> MADGPSPIRIVLWNDGGESLAAGVEDEEQQQVLHSFADLVGSAIDAVLELPQFRHVEAVTAEAEEDEPGLSIGFDAGSGDGEVDIDNLKGRLDIAGLLLGSAQLPEELAEVAAVEVTDEEEGTTELQFTDEGLVQQLQAVVKRAKLEKRYNDWVAGVAESLGPALDAAAGGVEVTEMPVDPYDVLQAVVAQLIRVAGVSPPAPSLFSRTGALVGGVLGAPRSAVRQVTKRLGRAQRLWWRLEDVVVDGSKLALRLAVKAARPVLVGFVLHRVLKTLDRSRQLEYRLARMGPEEAREAYYEAVLGKDWKQQLQADWDKALEDVDAGLVTDEINHEKRLMTAAQLRRLEVEEWDKQRMKNFYLASFGGLRWFDQMEQALHNPLFIESRGWTDPVQNWVGQNRTYMDDLPAGQYMAGVGNAAIRIKEAELKRKLTDVERAHVLARGGAVAGGLLPQQPTDPATLAVAVGGAFVPSVAGKR;> MGASQESELDFVPRLSFLPIEWRSIGSAFGLKDKSGAAANGRATFTVRQGVDAAELTSTGRVIDGQADVGASLKLNTLAIGVSASNITFHSGLDDPTAAAAQRSSLIPSLKLTAAKQFKRDNYIAVSYDLKHQKPELSACWTGEAGADRATLLVNVDPVMRSVKLAAAVRTPGPEWRKVLYNDETDLLEYPADDGARHTLYVQHEVRGRDLLHATRLGCRLDLGRLVNYVVDFVDYRIEENIPSFVWNVPLLPQLYSLLVPADNDEQVRHRITGWELDVSHDFARSGLLPVVAISKTSKKLLGGGTLTASYDAAAREAGVSLSRKGVSVGARVARAEGAAGGLSAGWGRPSIHVAVEPLGLLQ;> MQLGQLRQPLRACQDQRLTRGVPLARRQLVVVSNWNPLGGKGGGNAEQPGGEEPIQDELLKLLRGGWVLLSNLALFLVFSSFLHRSLNWFVQTELLVAVGAPQQAGERVVGKFFEAIEWVERNILGWKLPGDEEAEDATSKVYEVLQNYTPAEAAYSFAQLKYKDLTHKERELFHKAYALRHFERRDGRPGDVDAAELQAVKDRLDPLEADRRAYAAAKAAGRLDEYWAAPGREATYQRIVGAPRIAARQCEMASMLKGLQAVLPAMELLAQLQVAQFVYAASKASKSRQQDDFKLQLQTFYGNVLDEQCQLRCMLLNVQLPMALVTVFVPQYCFCLLDRVVLPRRECGSASTLGSLLRACGRPGSACHAGGCSAQRRDPLTI;> MQGLKATPGLRASSGRPTLRTARTALVVRAHASQPSSSNHAEQQECSSSGSGVSVNQPSALGRLGKFGLSSALSAFVLVPNFGGFGGNGGNRGGGGGGGGGGGSGGQGQPDGGLPLPLYELAEESSDEKEKQQKDDKRNWKNLVTDSEDLEEKPGERSGTNRCVEIVIEGWPDVGNLPTADELKDLLTVQEGHIFEKQDLLDDRRKLEIQYEDYIAEVEIRTEYVDGKSNHQRVVYKFTPHQFRGINAIDIKGAALMPASEVERICNECLPKQPYMVDIAVMDKVRNRIEQWYQSRGLPFCYVGFFDGMDDGILRANVTEAKIDNVSVRFVRPKLTGDSELEYSVYDEGKVVKADKIIEASGFQRGHHYHVEDGYDAMNSIFACGLLEDINIEPEQDPSDVNKINVKIRCEEVQPKSMELDLDWSFQLKNGIPSINRQSLIPGGSVEVSHENLFGNSESATLSLSASDWRNPSADLGFSVAYSEPFYKPHTTRNAQLFNTRKTSTIFTPGGESEVPPVFVDRFGLKGWTSQITGQDNKVEHALMLQLVSTLDENGQVVAKGTKVQRGYYADNGPPTTNSGNGRDLSLSYQGFFALDNVRFINGNQLGERMLFQVDQGLNPSISLPGGRKLGLSGGIYNRATASYTKFLEAPFLPKLTTEQLWKERKAPNTVVLHAKAGNALGDVAAYDYFSLGGPYSVRGYSHGEIGAARRFLELATEVRVPLKNYGLPGTAYGFVEYATDLGSGRELNGNPTEYYRKPGRGMSYGLGLKALGACRFEYARDCNAGTGTFLVNFGERF;> MGGGLPPKRSEVAESQPASSASSSAAAPAPAAETAGPKLPPRPAGLGLGGAGLLPSRGAAAAPSAGSATGTPAAAASSSLQQQQQQPAPPATQPAAHAAPAAPAGLGGAGLKPMLPPRPAAAAGAGAAGAAAAKPTPAPAPAAAPVPAAAPPPRPAMPNPAAGMSLPPRPVVAAAPPVLAAAGSDAVVDPSEDRRVQRVQRIAHDTRVRLIRAASRLGLAPRTDQVAQFLQAIERSERMVGAQHYKGSRRVDLLAAAEREARLAEEREGAAAEAVAGLRVKILVLGMTGTGKTELINSLLNRPAGSRTNAFREATRRVRVVRGDHNGIPLTFIDTPGLHASASRTADNRAILRAVRAAYRWHKPDYVFYVDRLDATRPGFGEMGLLGLITESLGAGVWRNTMAVLTHAHAARTAFGGQYDVNSRQRRNIVSQLLRQAAGDQQSRNPVFLADCHPACPTNSLGQPVILEGPTAVPWKQQLLVQLVGYKSYNVATSAFKDLAKAKAGKAAAGAAGGARGPQDIFKQMMRSRLPPMTFFVEQMSEGVLKPEGWATMETVAGLGEEVTEDEGAESFNHVYYRQMYELAVAGDPWAQREYAAMLRAYDKGCESYRASYEEADVDANVEYGVESYVVDPIDFGPSFDPEDMYSHRHAYAEAADAGVTVIPSQDYYGPEHDDPLNGIVFQYEAQPFSRHGWGGVPFDLTVCCEKDKTSLCLQGETHVSLVHSVPPFGPRHITQVTGSWEVLRPNIKDVMYQLEVDTFKDGLLGKSDHAGCGLMLARLGEGGDPRKGPTAVGVRLQDTLRVGPFKLEACASKVAVQGPTGGKEEGWGARAFVGYDWLPGLGMAFDFIQERTPEEGGKRLRGYGANFTYDWEALGAAFGMEVDYVAASESVFVSVNAFSGNDYRLGWLLLLPAVNYFKETVSSLWARLRGAGGGEGEEGEELEEEGEGEEGDDEEAMMMMAQEGDL;> MITFTFMSLVTSVKDYVEITHKLIEIEPLKNYTEFGAVFTYFIFSIGEFFKNFFSFSFLNNIWSIPIIIPDIASAMISEVSVLDGYFHNAFTFLETSVNTTTNPSLVIFEKFVIGIINSLFLILPTSTSHLITLRRFVMQGLEAGYMAGLGTLAGNFLWLASIILGWRFFVIPWLSLDIFRYLLGFVLLVKYIWDSSKERRMALEDLSKWKIFLLNFLLALTEQSCIYPFISNLSFGPDASILEGFPVDNYPQFLLIHGAYLLGILFGSFSLLQFTCWFWENPAFSIYLWITTKSSLKISTSSYYKILNFTFLYATMLCAIAS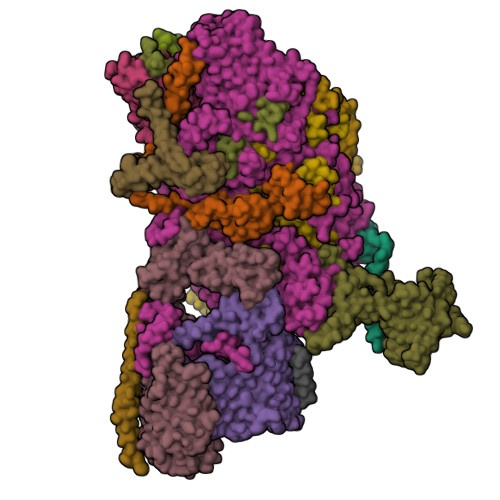IPYYGLDYTITNPIGLVPQDRILNQKKSQSDPDKLITETAFLNLNPTDKNSRIRDGVHARRERWKQRLIKYQAFDASTYDQGVYDFLTIEDLNYGFDRFWLRRKMRNHQIRFRLFPGPWMRSLKKQLNNPANPSLETSTKAASGPRVEFFRILFEQFYHPNFHDRAAMQTNPAEARNKFISTSPLASTESKKALNSTFSLGNINNSSTGIEGLVLTNTQATLLPTDLQTKRTIKPGLIYTNSALRKFVRNVNTRLNLKLLNSKETNLTTKYKSQFIYSKRWKSIFSKIQPLQNGTTRKSYQLFRNVAKQILVTPDAKSLKLITINQKLSLKERKLLELRTQYNNNSTLTTTAPLTLVRPLNVYLQKEEAFKRKLRYYGTMPMRKLTVGNQAPYFKALMKRGFYYYKPTLRWRKTLYVASLRRGFRKKSRKQRILVMPSNQQNFNNTLDNTKTNINQNNLANPLGGNEVPMYGADGENSLITKPTHSYTVLGKRASRYRHQIYKDVLQHWYYTPFNRLLMKFDVDAFINRQPKSHFLTKNEERALHIRRFLLSEHYDTLRWYTYMQHYKTMKTNIGGTKSFANRAYNQQFQGTFKKIRHLFAITPKQGDFYTLKFDQPLYNDNKLKDNLYFHEELLTDYYNGTNLQTNQTSNISVNSTTTFIDNSLRTTQLPVPSSSFDIVNQSSTLIGLTTMQNALRKNVVESTLTSLNSDGEAATSQPKLNFVYSELFVKLIKECKKRIHDQTFLKNYITHRIEKREQLNQEQTKELNKRLEKLKVWLNSDKGSISKLQNTPVQDPNISSPDKVLTTAMQKAVNESISLSGIMPSDKIKTTYGNLTNAYTIKTENAILTKLNVINQLTNNETTTQKNTLIKSIGVNKIQTVLQTIITNFKSSLYNQTQLLRVKTDKDLQWWRTKQRVITKRKSARKRDRFKKQIAVVNKKLAALSKKVETEKSNLYQTLYGNYEISDYLLRNVPTGSSAVIDSTVLRKKQDNQAYLPKETNNVQFNSFVDSNNNVWQTFFAKKLRKKISSKGRRYRSLSLARYLTATRKPRLVGLDNLTKIDNITTLQGAFITKEEKQDSLNLTIQRKQELTNSLKKSQIKKRSRHSWKKRSRHQFSRNHYKYRKRHTHGNGKLRVMNKKLKKFKATNELRQWWWNSFLPRYLSNLQVNNSTLTNKNVSFKPLSNTNSVPSTNMASPTTSRNLLDNLNSSNQISTSASMNQNIVTESVKVETNQVYLPEGEKSFDITSMTTTLPFYAGWDESLKKFVVTNRLLSRRDAGLSVNNNPQEINFTNPPIQGLNEGSFLYWQTEMPFNSYNIDQFITTNQSFYAPLGWRRFEFRHSILKTWVNNTKAGNNNIKKKTLIISLKNLQPLKSSQQKQNQIKTKKLVARRIKKRYKLLKQMPNQLMYSPTGPLLTEVLPSHYISVFDQQYRLPRNRYLKRNPLKTLKKTTLLALMDSSKQTNGVNKEFTLRKRVKPRRKYHRKRFIKKDGLIFPRRTKFNTNTTLTGNALITNNVNSIEEDDLRWRPSSRTKQKRKDNTRSSAASKTKSNKRVKTNPLRLRQLRRREFQQVLKPLQRYIPQNGGFTWPGDYLRLEIVEMPKLKSINIKKTSLKQKINVQPVGIMPRKYLIEKHNIKVLKKKLSQAYSTQQLTKVVQEYKNLIQNSPPAI;> MSALLSQASGFSGLALGSSASSKRLCKPLCRRPAVCVQAAHRPASAVSSGVPSTGFGPVSPLQRRPTLPTRKLVVASSQSGGRAEDAEKQDWKFGRNEGPMTWPWKLMCAILYMLPWVDVTEKTVYFVERFPAFVWTEYFSEPFEHWYNIHEYAPLFIFFATYLGIVRNKKIPHVARYHVMMGVMLDIVAMILIVTEENLPTGVLWTPWSDLFYALMFWFIFLLVIYCLFFCFLGWYCEIPLISEGVYLQIEQAEQLGQ;> MDEEPPFNLALNVYKGPASIPHASAEVFGAFFLATNTALLAHMFPGKLFGSELHVRKWDPDYLASCCNEQGMRREALSGKKPNLWLLGGGPRLVNDSWERMWWNNLHWKRWKVPRTGPAFPQDMYWQ;> MATCAAVSLATAVFQVAAKYVNKARDAVASALPSPSNIDGVQQDWRQQVKELKKHTRVLGFVLPLAKAFAAESLTSVYARTFERAAFGFAKMYLFCLFMRVLLSWFPSIDWNSQPWAFLRLITEPYLQIYRGILPPLFGQLDFTPLFGFLILQDVVELMSPVYTLGHAKDTSMFWTTTDIMCYFDGH;> MASKKGTDAPAALTDPLKEDPTVIRDEAQFPEPSLYFKVFESEAGEPEAKIRADVNKLYDRWIEKYGRRWPEDGINTEDMVWLAEEANKRKRAKPRPRGTVAAEKTEYEDEFMPDPTVGAPVSAADAAKAARRAKKDRKKKKAAGGAEQPAGPRTNYEKTVAGGKWVTDEFESADYEAGNLEKLWDMYLWDREGKPTMMPDTPAAQQEGEESEDFDDFYTAYRPRDVDSEEAREAVWATDEFESDEDNTESEWAPEYVGAGLGLVAEDPLNPQYSLRHSNHPLAPFPGEPLKWASYVYPDFTTFEGLSKQSIPHGMGVMTFGTGTGAGFAMSQTRYGDKYEGEFQAGYAHGLGQFTSEASGEVYIGEFFAGQRHGCGMTLDMKPYFYLLERGVDPVEAYRRTAGAIMKNVEVRTWYRGNKLGDAKEDEVVEINVLKDELDDPFEIALRNSLHDAKLRKWKAMSPQDKAMDRIVSIIERVQRRNPGRFGAYYREDEKGRVRPVLDSDGADTDFDSVDMIQGVDTDGDLGPGWEGATDSEENPMDPRIRELMAAEGMDDKLEDEGFKDTVLGSAIINPYTGLDMKTYLDGKERHQAELVSVYKASREGRKYLNKVRKDKGGAAKDDESSYVEDDAASGHPGALLSREAEDDRLARLYEQAGVSKEDERRVEGLAARWRRLLAADEEEVLGGAVGAFRRPGNPLAANDSDTGFETESDMMEMCDIPEILGTVQEARQIVERARMWRFKPYGEVGLRMAQDANGSPVSLMQEPLHYPHGTKFMAPGPLGLCHAVPDDPSLRQEMAKVAHNYAAIYRMYNFDWDPEPGTVQYKIDQRIRRAQELRNNAMARYLAAADEVLRDGAAPAGEGDQALLLASTSTGAPEAFDGQGNASGSGSSSALSSRGGSMFASMTLSRPAPMAGVVSLGRAARVVLGAFADAAKSVPMARPRLARPSGRRQ;> MSEPGAGPSDGQVVTRKIRLHKVMRPLDESSPSSQEQHMDRRLAEILPAIADLPVPGPSGAGGSPADARAVEMRRLRGTQQELAQMEAMELATLFDMSKPHPLDNAAPATPWKGELRPVPRKIVLSPYQYEMINYQRMLMRKNIWYYRDRMNVPRGPCPLHVVKEAWVSGIVDENTLFWGHGLYDWLPAKNIKLLLPMVRTPEVRFATWIKRTFSLKPSLNRIREQRKEHRDPQEASLQVELMR;> MAQPPRPAEEYDDDVQEDEDELKEGELDDDESHEAASEGGEAAAGDEEAEDDEQDEEDGDEDSQPWAGLNRLPERDDMLDILNELRAEGRKQLTVLLLGKSSVGKSSLINSLLGEAVVRVQAFKLQADTDITTTVVRQVAVGNSEVDGFRLKLIDTCGLEDPEAGDTVNLGALSKIAEDVRGVGIDVVLYCDRLDLYRVDPLDKAIIDAISSTFGRGIWRRTVVALTHANLVQTPPGTDYDSFVNGRVRLIRGAVRGPLFFRPSLPVALVENSETCPVSSESGFRVLPDGEPWLVALVSQLVDMAAARRRPYKYHPRLSSKPSHRFRWLLPVAIAAEVLFYRRFLHPRLDDNQRRVEREEERVWALRGQQRRALGLHRPHRPDKDAAWRLEQMYDDD;> MSSDVQAKLSGLLGDIGVKCTLAFAGTVAAGAAIVVPSGKQVEAASLDIYGRPPSQLLPNERRAAEFAAGHRRWKGFVDNSIYSWTRTLPGHDNPIVNPYKGPRRPQRPQQKLEEEVEAAAKQE;> AAAAAFAAFAGFAFAAFAAAG>[4x]MVPTQAHPEWYKSAVFYELSVRTFQDGNGDGKGDFPGLTSRLDYLKNLGVDCLWLLPWFPSPLRDDGYDVADYRGIHPDLGTLDDFKVFLREAHARGLWVIGDLVTNHTSSDHPWFQAARRGPTLPDGSPNEYHDYYVWSDEGKEYADTRIIFTDTEVSNWTLDEQAGKYYWHRFFASQPDLNYDNPKVVEELHGAARFWLDLGLDGFRVDAVPYLIEREGTSCENLPETHEILKGFRAMVDREYPGRLLLAEAAQWPEEVVEYFGTEAEPEFHMCFNFPVMPRLYMSLKREDTSSIREIMGRLPKIPSFGQWCIFLRNHDELTLEMVTDDERAFMYAAYAPDARMKINVGIRRRLAPLLDNDRRRIELLNTVLLALPGSPVLYYGDEIGMGDDLGLPDRNGVRTPMQWNAGTSGGFSTAQPSDCFFPPIQDPVYGFGRVNVQSQLQDPSSLLKWTARQLELRRAHPAFAHGDLTFIETGNPAILAFTRQYDGETLLIVSNFAGNAQAGLLDLAPFVGRAPVTLSGASPLPVVTGNGQYPVVMGKYDYYWLRLNSRVDKLAAALEHHHHHH

Trehalose synthase (TS) catalyzes the reversible conversion of the inexpensive maltose into trehalose in the absence of any coenzyme. DrTS consists of a catalytic (β/α)8 barrel, subdomain B, a C-terminal β domain and two TS-unique subdomains (S7 and S8). Domain C and sub­domain S8 contribute to dimer formation, while subdomains B and S7 serve as a gateway for the opening and closing of the active site. In the present study, we have determined crystal structures of the wild type and the N253A mutant of TS from Deinococcus radiodurans (DrTS) that reveal a closed conformation for intramolecular isomerization.

The four or eight subunits in each asymmetric unit did not display significant differences, with root-mean-square deviations of 0.3–0.4 Å for all Cα atoms. The peak was assigned as a Tris from the crystallization solution, which contained 300 mM Tris–HCl, forming hydrogen bonds to Asp63, His106, Asp209, Glu251 and Arg398. In addition, the interaction networks between subdomains B and S7 seal the active-site entrance. Disruption of such networks through the replacement of Arg148 and Asn253 with alanine resulted in a decrease in isomerase activity by 8–9-fold and an increased hydrolase activity by 1.5–1.8-fold. The N253A structure showed a small pore created for water entry. In the N253A mutant, disruption of the interaction between Asn253 and Glu324 results in movement of the Glu324 side chain to create a small pore for solvent entry to the active site. This may explain why the N253A mutant has ∼11% of the isomerase activity and ∼180% of the hydrolase activity of the wild type. Similar to N253A, the R148A mutant shows ∼12% of the isomerase activity and ∼150% of the hydrolase activity of the wild type, suggesting that a small pore for water entry may also be present when Arg148 is replaced by alanine.> GUUAAUCAUGCUCGGGUAAUCGCUGCGGCCGGUUUCGGCCGUAGAGGAAAGUCCAUGCUCGCACGGUGCUGAGAUGCCCGUAGUGUUCGUGCCUAGCGAAUCCAUAAGCUAGGGCAGCCUGGCUUCGGCUGGGCUGACGGCGGGGAAAGAACCUACGUCCGGCUGGGAUAUGGUUCG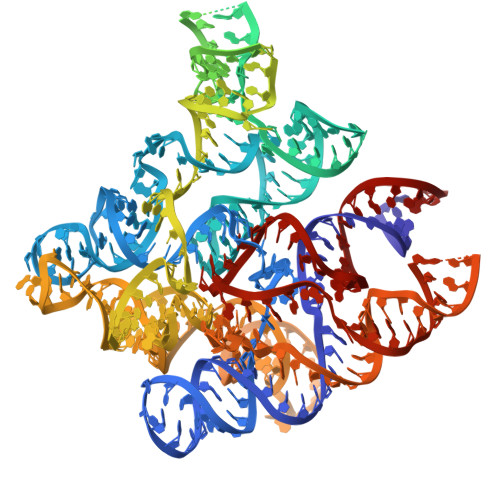AUUACCCUGAAAGUGCCACAGUGACGGAGCUCUAAGGGAAACCUUAGAGGUGGAACGCGGUAAACCCCACGAGCGAGAAACCCAAAUGAUGGUAGGGGCACCUUCCCGAAGGAAAUGAACGGAGGGAAGGACAGGCGGCGCAUGCAGCCUGUAGAUAGAUGAUUACCGCCGGAGUACGAGGCGCAAAGCCGCUUGCAGUACGAAGGUACAGAACAUGGCUUAUAGAGCAUGAUUAACGUC>MTKKMRRVGKYEVGRTIGEGTFAKVKFARNTDTGDNVAIKIMAKSTILKNRMVDQIKREISIMKIVRHPNIVRLYEVLASKSKIYIVLEFVTGGELFDRIVHKGRLKEDESRKYFQQLVDAVAHCHSKGVYHRDLKPENLLLDTNGNLKVSDFGLSALPQEGVELLNDTCGTPNYVAPEVLSGQGYDGSAADIWSCGVILFVILAGYLPFSETDLPGLYRKINAAEFDCPPWFSAEVKFLIHRILDPNPKTRIQIQGIKKDPWFRKNYVPIRAREEEEVNLDDIRAVFDGIEGSYVAENVERNDEGPLMMNAFEMITLSQGLNLSALFDRRQDFVKRQTRFVSRREPSEIIANIEAVANSMGFKSHTRNFKTRLEGLSSIKAGQLAVVIEIYEVAPSLFMVDVRKAAGETLEYHKFYKKLCSKLENIIWRATEG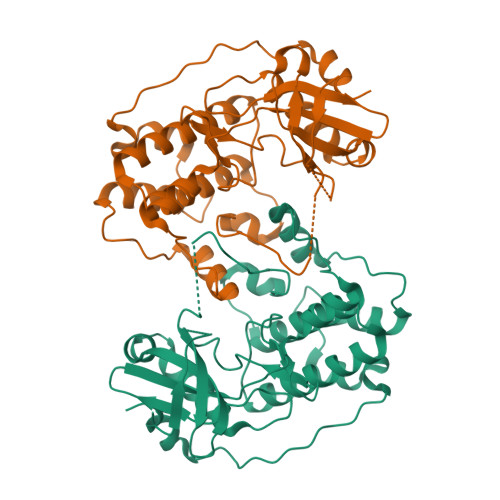IPKSEILRTITF[4x]> AQSVPYGVSQIKAPALHSQGYTGSNVKVAVIDSGIDSSHPDLKVAGGASFVPSETNPFQDNNSHGTHVAGTVAALNNSIGVLGVAPSASLYAVKVLGADGSGQYSWIINGIEWAIANNMDVINMSLGGPSGSAALKAAVDKAVASGVVVVAAAGNEGTSGSSSTVGYPGKYPSVIAVGAVDS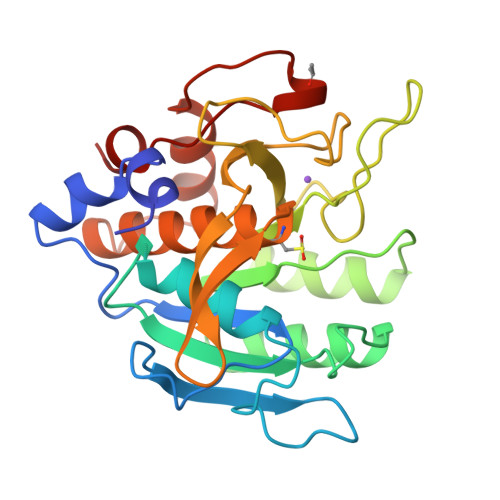SNQRASFSSVGPELDVMAPGVSIQSTLPGNKYGAKSGTCMASPHVAGAAALILSKHPNWTNTQVRSSLENTTTKLGDSFYYGKGLINVQAAAQ>MIKPLGDRVVVKRIEEEPKTKGGIVLPDTAKEKPQKGKVIAVGTGRVLENGQRVPLEVKEGDIVVFAKYGGTEIEIDGEEYVILSERDLLA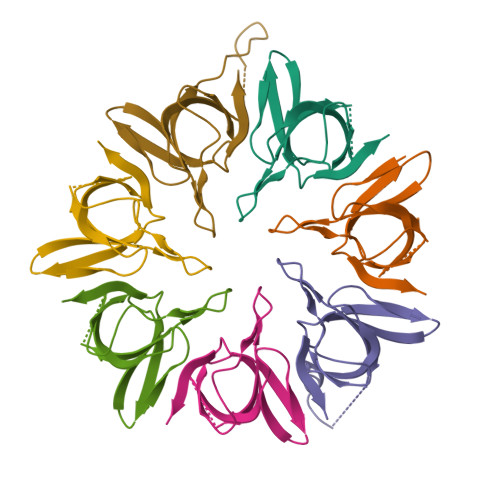VLQ[7x]> SANEDMPVERILEAELAVEPKTETYVEANMGLNPSSPNDPVTNICQAADK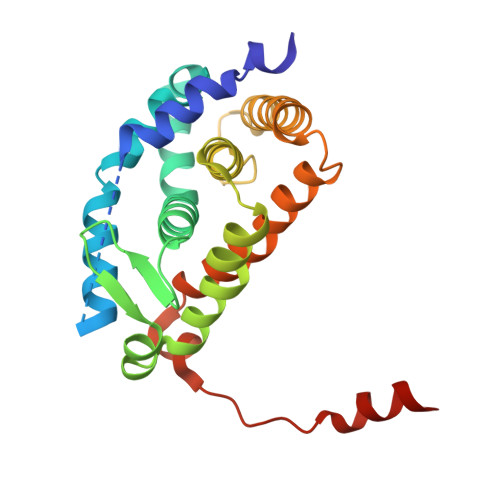QLFTLVEWAKRIPHFSELPLDDQVILLRAGWNELLIASFSHRSIAVKDGILLATGLHVHRNSAHSAGVGAIFDRVLTELVSKMRDMQMDKTELGCLRAIVLFNPDSKGLSNPAEVEALREKVYASLEAYCKHKYPEQPGRFAKLLLRLPALRSIGLKCLEHLFFFKLIGDTPIDTFLMEMLEAPHQMT>MAAVTLHLRAETKPLEARAALTPTTVKKLIAKGFKIYVEDSPQSTFNIN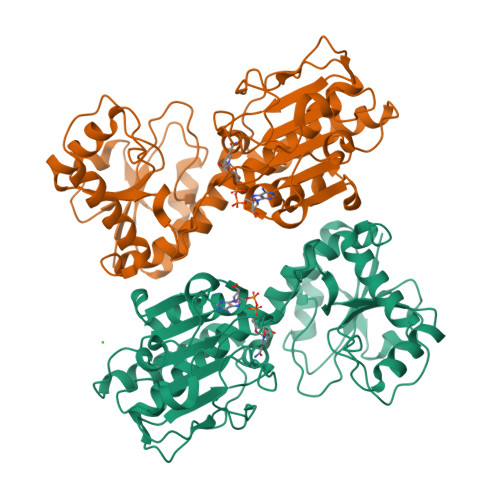EYRQAGAIIVPAGSWKTAPRDRIIIGLKEMPETDTFPLVHEHIQFAHCYKDQAGWQNVLMRFIKGHGTLYDLEFLENDQGRRVAAFGFYAGFAGAALGVRDWAFKQTHSDDEDLPAVSPYPNEKALVKDVTKDYKEALATGARKPTVLIIGALGRSGSGAIDLLHKVGIPDANILKWDIKETSRGGPFDEIPQADIFINCIYLSKPIAPFTNMEKLNNPNRRLRTVVDVSADTTNPHNPIPIYTVATVFNKPTVLVPTTAGPKLSVISIDHLPSLLPREASEFFSHDLLPSLELLPQRKTAPVWVRAKKLFDRHCARVKRSSRL[2x]> GGUGGUCUGAUGAGGCC;> GCCGAAACUCGUAAGAGUCAC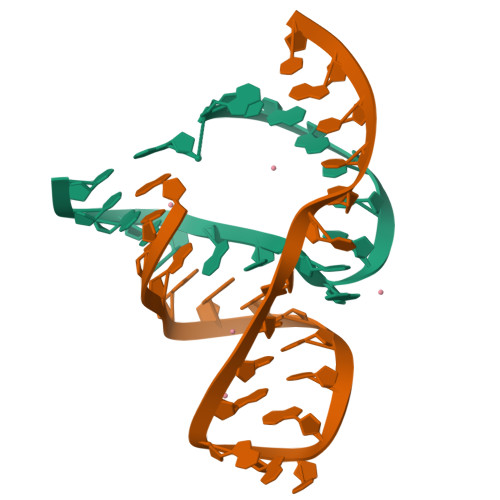CAC>[3x]MFTGIVQ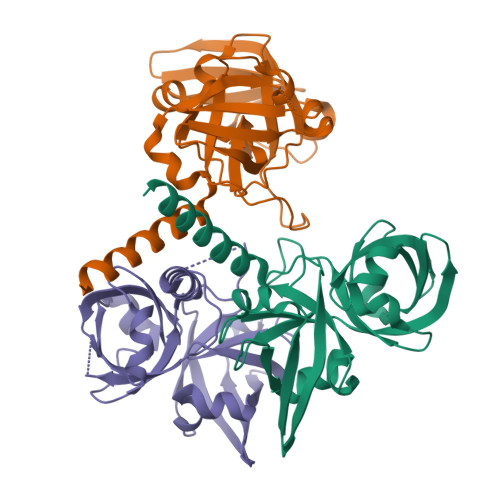GTAKLVSIDEKPNFRTHVVELPDHMLDGLETGASVAHNGCCLTVTEINGNHVSFDLMKETLRITNLGDLKVGDWVNVERAAKFSDEIGGHLMSGHIMTTAEVAKILTSENNRQIWFKVQDSQLMKYILYKGFIGIDGISLTVGEVTPTRFCVHLIPETLERTTLGKKKLGARVNIEIDPQTQAVVDTVERVLAARENAMNQPGTEA>[3x]XEVE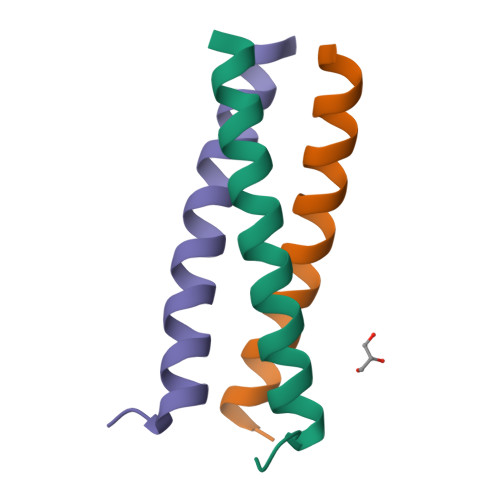ALEKKVEALEWKVQKLEKKVEALEHGWDGR>[4x]MDYNLALDKAIQKLHDEGRYRTFIDIEREKGAFPKAQWNRPDGGKQDITVWCGNDYLGMGQHPVVLAAMHEALEAVGAGSGGTRNISGTTAYHRRLEAEIAGLHQKEAALVFSSAYNANDATLSTLRVLFPGLIIYSDSLNHASMIEGIKRNAGPKRIFRHNDVAHLRELIAADDPAAPKLIAFESVYSMDGDFGPIKEICDIAE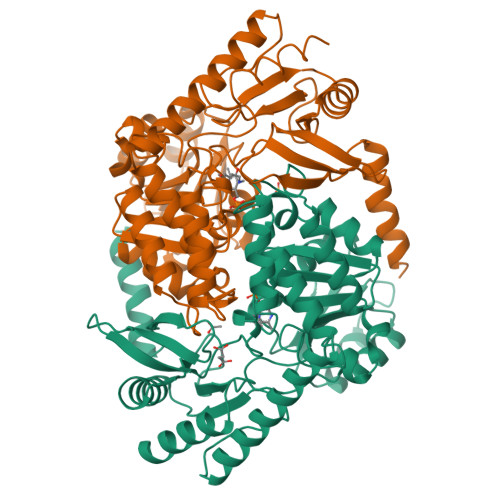EFGALTYIDEVHAVGMYGPRGAGVAERDGLMHRIDIFNGTLAKAYGVFGGYIAASARMVDAVRSYAPGFIFSTSLPPAIAAGAQASIAFLKTAEGQKLRDAQQMHAKVLKMRLKALGMPIIDHGSHIVPVVIGDPVHTKAVSDMLLSDYGVYVQPINFPTVPRGTERLRFTPSPVHDLKQIDGLVHAMDLLWARCA N'-[(1E)-(3,5-DIBROMO-2,4-DIHYDROXYPHENYL)METHYLENE]NICOTINOHYDRAZIDE | C13 H9 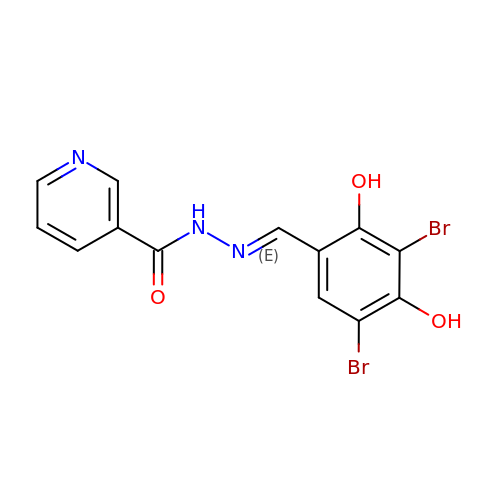Br2 N3 O3 | PYVJEAZDEZTGIS-UBKPWBPPSA-N>[4x]MNRLPSSASALACSAHALNLIEKRTLDHEE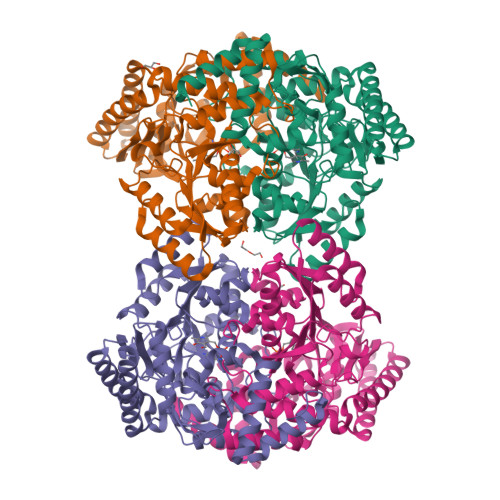MKALNREVIEYFKEHVNPGFLEYRKSVTAGGDYGAVEWQAGSLNTLVDTQGQEFIDCLGGFGIFNVGHRNPVVVSAVQNQLAKQPLHSQELLDPLRAMLAKTLAALTPGKLKYSFFCNSGTESVEAALKLAKAYQSPRGKFTFIATSGAFHGKSLGALSATAKSTFRKPFMPLLPGFRHVPFGNIEAMRTALNECKKTGDDVAAVILEPIQGEGGVILPPPGYLTAVRKLCDEFGALMILDEVQTGMGRTGKMFACEHENVQPDILCLAKALGGGVMPIGATIATEEVFSVLFDNPFLHTTTFGGNPLACAAALATINVLLEQNLPAQAEQKGDMLLDGFRQLAREYPDLVQEARGKGMLMAIEFVDNEIGYNFASEMFRQRVLVAGTLNNAKTIRIEPPLTLTIEQCELVIKAARKALAAMRVSVEEALEHHHHHH>[2x]GTIYPRNPAMYSEEARLKSFQNWPDYAHLTPRELASAGLYYTGI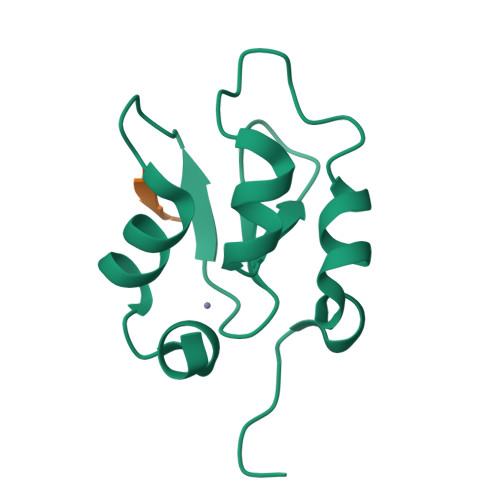GDQVQCFACGGKLKNWEPGDRAWSEHRRHFPNCFFVLGRNLN;> AIAV>[4x]TGRLNIAVLPTIAP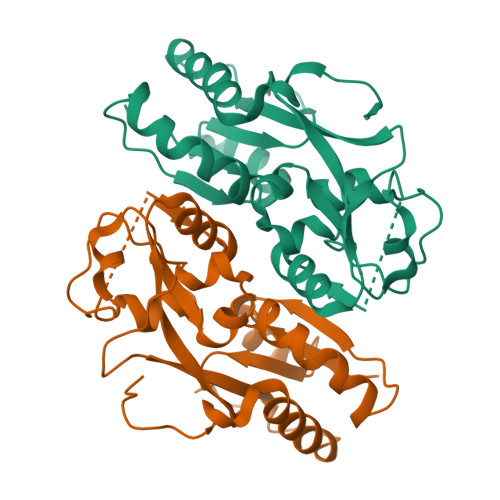YLLPRVFPIWKKELAGLEIHVSEMQTSRCLASLLSGEIDMAIIASKAETEGLEDDLLYYEEFLGYVSRCEPLFEQDVIRTTEVNPHRLWLLDEGHCFRDQLVRFCQMKGLHERQTAYSGGSMEAFMRLVESGQGITFIPQLTVEQLSPSQKELVRPFGMPRPVREVRLAVRQDYSRRKLREQLIGLLRSAVPSDMHKLQTGQHLAHHHH4-[(4-methoxypyrimidin-2-yl)amino]-2-[(3-methylbut-2-en-1-yl)oxy]benzonitrile 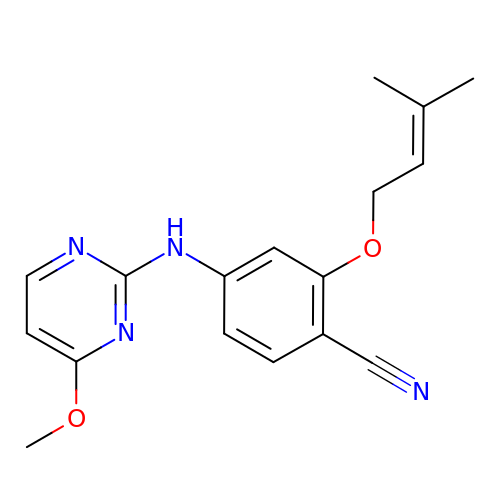| C17 H18 N4 O2 | VFPQRVJYEMSZLR-UHFFFAOYSA-N> MFAWWGRTVYQFRYIVIGVMVALCLGGGVYGISLGNHVTQSGFYDEGSQSVAASLIGDEVYGRDRTSHVVAILTPPDDKKVTDKAWQKKVTEELDQVVKDHEDQIVGWVGWLKAPDTTDPTVSAMKTQDLRHTFISIPLQGDDDDEILKNYQVVEPELQQVNGGDIRLAGLNPLASELTGTIGEDQKRAEVAAIPLVAVVLFFVFGTVIAAALPAIIGGLAIAGALGIMRLVAEFTPVHFFAQPVVTLIGLGIAIDYGLFIVSRFREEIAEGYDTEAAVRRTVMTSGRTVVFSAVIIVASSVPLLLFPQGFLKSITYAIIASVMLAAILSITVLAAALAILGPRVDALGVTTLLKIPFLANWQFSRRIIDWFAEKTQKTKTREEVERGFWGRLVNVVMKRPIAFAAPILVVMVLLIIPLGQLSLGGISEKYLPPDNAVRQSQEQFDKLFPGFRTEPLTLVMKREDGEPITDAQIADMRAKALTVSGFTDPDNDPEKMWKERPANDSGSKDPSVRVIQNGLENRNDAAKKIDELRALQPPHGIEVFVGGTPALEQDSIHSLFDKLPLMALILIVTTTVLMFLAFGSVVLPIKAALMSALTLGSTMGILTWMFVDGHGSGLMNYTPQPLMAPMIGLIIAVIWGLSTDYEVFLVSRMVEARERGMSTAEAIRIGTATTGRLITGAALILAVVAGAFVFSDLVMMKYLAFGLLIALLLDATIIRMFLVPAVMKLLGDDCWWAPRWMKRVQEKLGLGETELPDERKRPTVRESETDQRALVGVGAPPPPPRPHDPTHPAPEPVRPMPPMRSNAPSAAGTARISTPPQPPQPPQAPAQQAGDEPATTRFAMARNAVRNAVNSAVHGGAGSAAAPTERAPRPGGPAQPPAPPQREEREIESWLGALRGPAPAKNVPQPPAQPQRPSTDTTRAMPPQGRPPAGPADRGNENAPTTAFSAQRPPNGGAPADATTAIPTPPQREQEPSTEKLNTREDAPEDPETKRRGGGMSAQDLLRREGRLHHHHHH

The mycobacterial membrane protein large 3 (MmpL3) transporter is essential and required for shuttling the lipid trehalose monomycolate (TMM), a precursor of mycolic acid (MA)-containing trehalose dimycolate (TDM) and mycolyl arabinogalactan peptidoglycan (mAGP), in Mycobacterium species, including Mycobacterium tuberculosis and Mycobacterium smegmatis. A detailed analysis suggested that MmpL3 is a TMM flippase that is absolutely essential for transporting TMMs across the cell membrane. MmpL3 consists of 12 transmembrane helices (TMs 1 to 12) and 2 periplasmic subdomains (PDs 1 and 2). Our structural data are in line with MD simulations that indicate the major conformational change of the transporter is located at the periplasmic subdomain PD2, where this movement can easily be interpreted as a rigid body rotational motion of PD2 in relation to the PD1 subdomain.

We then reconstituted the delipidated, purified MmpL3 transporter into lipidic nanodiscs. The structure of MmpL3-ND was solved using single-particle cryo-EM. The reconstituted sample led to a cryo-EM map at a nominal resolution of 3.65 Å. Density modification allowed us to improve the resolution of the map to 3.00 Å. The cryo-EM structure of MmpL3-ND indicates a monomeric molecule that spans the inner membrane and protrudes into the periplasm. Overall, the conformation of the cryo-EM structure of MmpL3-ND is comparable to that of the X-ray structure of MmpL3773-PE, although there are some conformational differences between these 2 structures. The conformation of MmpL3-ND is distinct in that the gap between subdomains PD1 and PD2 is larger when compared with that of MmpL3773-PE. The volume of the periplasmic central cavity formed between PD1 and PD2 was measured to be 1,794 Å3 in MmpL3-ND. Based on the structural information, the increased volume of the periplasmic central cavity of MmpL3-ND is in part caused by the increased separation of PD1 and PD2.> PSLLHKYMGIFFSTMSSEELLGSLDSFDAREDDIFLVSYPKSGTHWLAEVIERIPDAGIT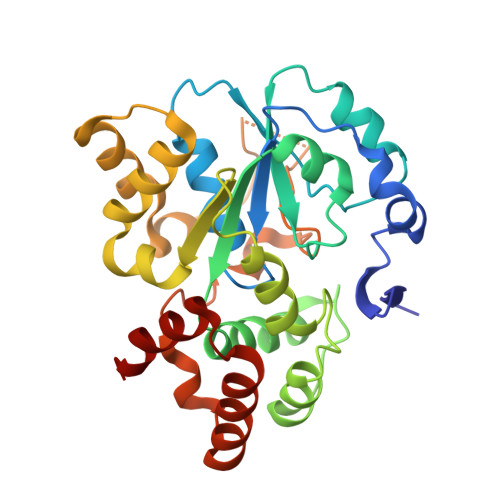LTSPIELGDISKFEELKRIPKRRAIPTHLNYEMLPVTVKQKQCKIIYIVRNPKDTAVSMFHYYRDNPNLPSTETWAAFLELFLKGDVVYGSWFDHVLSWEEHKNDKNVLFIFYEEMKKDFVKSLKKITAFLGIDVNDSEMAKIARSTSFSEMKSNAAKENCDPNHVICALTSDRNLVFRKGVVGDWINYFTPKQNRGFDELFTEKMRNSDVGRCLKEYAHSA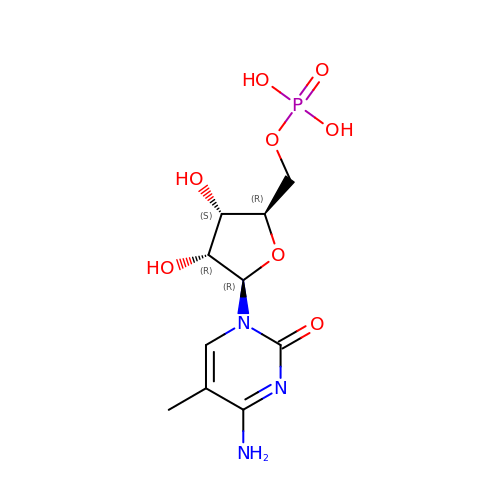5-METHYLCYTIDINE-5'-MONOPHOSPHATE | C10 H16 N3 O8 P | NJQONZSFUKNYOY-JXOAFFINSA-N> MAFAQRIITSNSAGDQEFTFTFDYIKEEHIKVFVNFVEKAQGTGSNEFQVITNTTPKKISLNTGLSADNTRVEIRRVSSLSTPL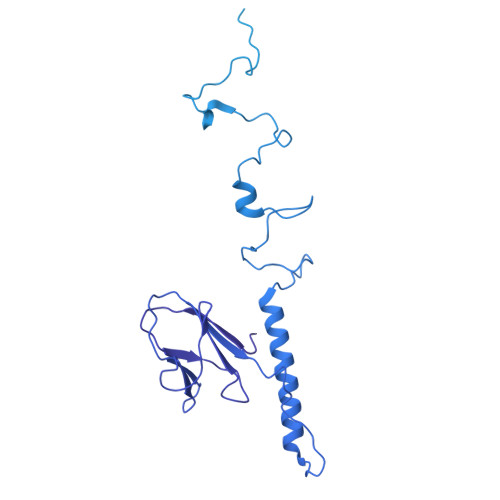VDFADGSTLTAADLDTAEKQSLFIDQELDDALKQGISIDTSTGVPTLNSQRLSNVSDPVNAQDAVTKAYLERSGSITSTQILNGTIVDADINASAAIAKSKLAALNIVNADVNASAAIAGSKLADASIAYTKIQNVSATNRILGRDSSGAGVIEEITPANLRTMINVEDGATADQSAAEIRTLVESASDSNVFTDADHTKLNAIEASADVTDATNVDAAGAVMNSDTSTAAMQFVIDEDTFGSNLDTKVPTQQSVKAYITATSQPLDSELSQLAGMQSGTASKLADSTALTADIADLNQLDGMAKETSITNSNTKFPTSAAVVNFVANQIAPVGGLEVIADEDSFPATQPVSGVVISISNADGLVINNAGEASNARTVGSGSDNVTIKNFPASLRNQTLAPNLGLLVSSTGASQEYNYHKLLAKETDVLQLSDDINDFNNRYRVENTLPAANDSSNHDGDLVYAKEEKKIYVYSGDYNGTPVGSFGEVQSIGNFFISTLSPAFNGSLQDFTITNAPSNAQQIILSINGVIQKPNSGTSTPSEGFALSGSTIKLAAAPPSGADYFAIVLGSTVNIGTPSNNTVTSSILQNGSVIEAKLGSGAVTRTKLNLVSTSSAPGLEVKGDGSSDGYLQLNCSQNSHGIKLKSPPHSAGQSYTLTFPSNIVSGQFLTTDANGNLSWAAVVTDLVNDTSPQLGGNLDCNDKNILLNDSSGSANNRIRLGASQDFALFHNGTINIIEAVSGDLHLRLNGSEEGIIVKQNGAVELYYDNSKKFHTSSVGATVTGNLFLSGGYINLNDNYSYGMGSGNRAQLYHSGNHQYLLNTVGNMYFQPKSGENGIVIIPDDAVELYHNNVKRLETTSGGVTVSGSVTATGHLFVGANTHYLYFTSTAGYSPRIGNADGGTGVNMTFHTNNTMRMMLQNDGHLRPASNNTYDLGTSSDRWRNVYTNDLNLSNEGGANDVDGTWGSYTIQEGAEDLFLINKRTSKKYKFNLTEVS> EVRPFLDVYQRSACQTRETLVSILQEHPDEISDIFRPSCVAVLRCSGCCTDESMKCTPVGKHTADIQIMRMNPRTHSSKMEVMKFMEHTACECRPA;> QVRPFLDVYQRSACQTRETLVSILQEHPDEISDIFRPSCVAVL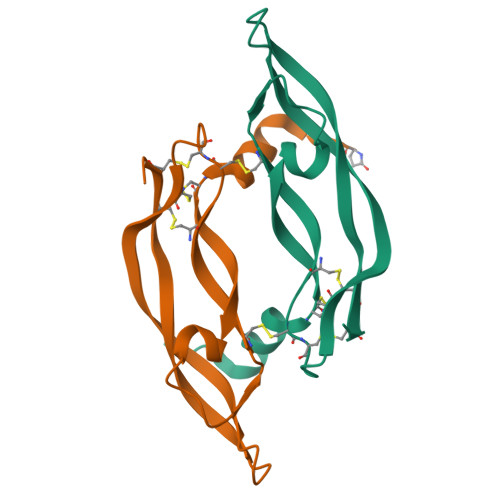RCSGCCTDESMKCTPVGKHTADIQIMRMNPRTHSSKMEVMKFMEHTACECRPA> MAHHHHHHVGTGSNDDDDKSPDPMLLSRKIRDYGAKYRGKEIKMSTEINSFLNLRNTIEMRIGSYTAFGVIYSISMDSLKLIFQEDTVLPALAKNKNLGSIQLKKNSDSKSSAAFFPFLSVKLLSASAYSSLNKEYNLLTLEFLSPAPEEIAIKVGKLLDLKLGQNQRIHE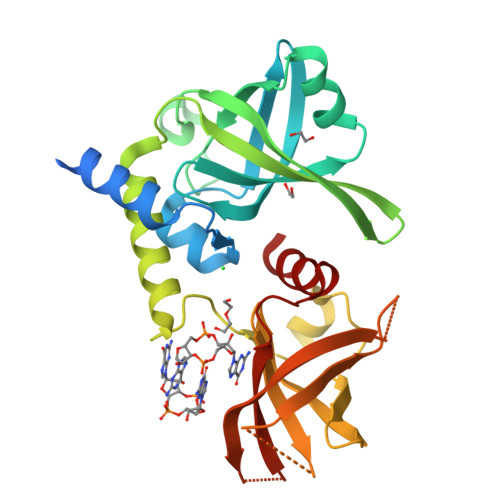RIIIDKDSIRKLKIDSDKAFIKFNGAKHKCLIKDLSYGGALVISSFDYGDVEEDAIDLIFSFEFIDGEIFIEGKSKSLSVIQTPSGKVFALGIAFDEDKIPLEYTMLIHDYFN>MAHHHHHHVDDDDKMVHHDGFQTVKATIDWEHPMFK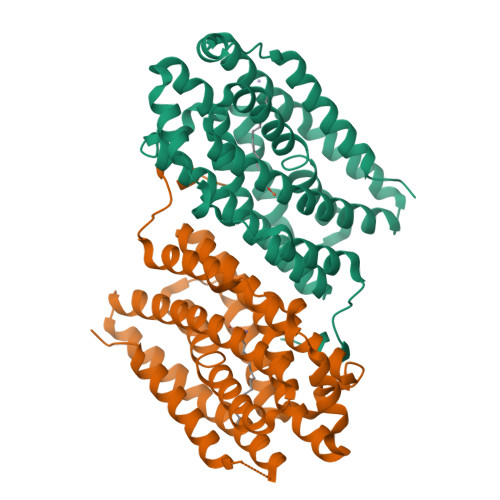LYEKAKRNGKWNPADIDFSQDQKDFASLTSEEKISALPLVAGFSAGEEAATLDILPMAHALARQGRLEDVLFLTTFMHDEAKHVEMFSRWQQAVGIGQMDLSVFHNDHYKRIFYEALPEAMNRLYADDSPEAVIRAATVYNMIVEGTLAESGYYTFRQIYKKAGLFPGLLQGIDYLNMDEGRHIQFGIYTIQRIVNEDERYYELFIRYMDELWPHVIGYVDYLTELGKRQQQLARTYALEIDYDLLRHYVIKQFNLRKKQISRTKRVDVVEGLEKTAAES[2x]> GIDPFTQRNAIREDLDNYLNEMGEVTADNIQTWLSGRILLIENAAQNIAINPEPAAVASLLEQKALTSTFMASYLGDATGHFTIRPDAKMPDGFDPRVRPWYKGAESSSTSTLTEPYIDAATGQTIISIATAAKKAGQSVGVVGGDLSLQTLINTLSARDFSGMGYAFLVSADGKILVHPDKALVMKSLKEAYP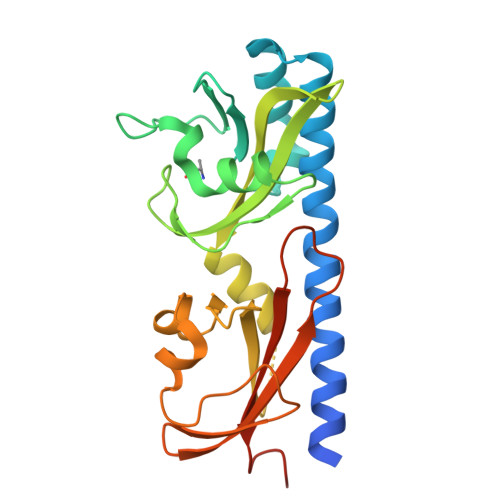QDTPRISSDFSEVTVDGKTRIVNFTPIKGLPSVNWYIGLSVDKDKAFSMLSEFRTS>[8x]MATERTLSIIKPDAVAKNV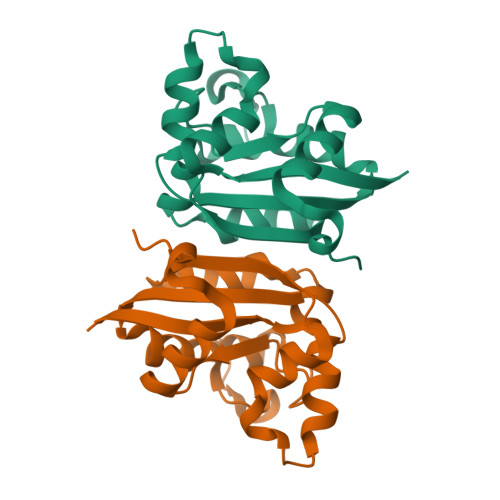IGEIESRFEKAGLKIVAAKMLQLSQEQAEGFYAEHKERPFFGDLVGFMTSGPVVVQVLEGENAIAANRDLMGATNPKEAEAGTIRADYAQSIDANAVHGSDSPESAAREIAYFFAESEICSR Antifreeze proteins (AFPs) are a class of IBPs that have been documented in a number of cold-tolerant fish, insect, bacterial, fungal, and plant species, and this phenotype permits them to prevent and/or control ice crystal formation. Previously we examined the expression, ice binding affinity, and effect on cell viability during freeze-thaw cycling of a bacterial protein. This 54 kDa AFP (IBPv) was secreted by a bacterium within the family Flavobacteriaceae (strain 3519–10) that was isolated from a depth of ~3.5 km in the Vostok Ice Core. Based on the recombinant IBPv exhibiting TH of 2.2°C at a concentration of 53μM, it is categorized as a hyperactive AFP. According to primary sequence, IBPv was predicted to consist of two separate ice binding domains.

Each domain contains a six-loop right-handed β-helix (solenoid) with a triangular cross section, and an α-helix, which runs parallel on one side of the β-helix. However, no electron density was observed for the last 88 amino acids of the C-terminus. Each domain contains one intra-domain disulfide bond, namely C165-C226 in domain A and C244-C443 in domain B. Sometimes the ice binding regions also consist of well aligned side chains and even well aligned water molecules. In the IBPv structure, one flat plane was observed on the same surface for each domain as shown in Fig 1B and Fig 2, and they were not at the protein-protein contacts in the crystal. Site-directed mutagenesis confirmed that the proposed ice binding site for each domain is located at the same region on the β-helix for IBPv. Each domain of IBPv has two rows of water molecules on the IBS that form hydrogen bonds with the protein backbone, and more water molecules are found in the IBS of domain B compared to domain A. In the crystal structure of IBPv, a layer of ordered water molecules forms a water network that consists of several pentagonal and hexagonal ring on the IBS of domain B. However, no such water network is observed on the IBS of domain A, which is the weaker one in ice binding activity of the two domains, suggesting that the presence of water network is correlated with the ice binding activity and thus supporting the anchored clathrate water binding mechanism. Close molecular comparison of the two domains revealed that the bulky side chain of Leu 174 on the IBS of domain A may account for its inferior antifreeze activity.

>[2x]MQAPTLGAAANFALFTTAGAVTNTGLSHITGDVGTNNAASTNFGNVDGVMQDSNGATSAAAADLLIAYNLLNAAIPTATLAPLLGNGTTLTAGNYFIGQGASLSGTLTLDGGGNSNSVFIFKIQGALSSAANTQVLLTNGALACNVFWKVEGLVDLATNTVMKGNVVANNAAIVLQSGVSLEGRALSTTGAITVTGVTVRKPILCGSAVLTGPVAPNLGTVVCYTIFSGNGALTNAGITYVTGDVGTNVGLTTGFQADNVNGTIHSNPDTSTAQAALDLNNAYTYLNTLPTDIELLYPAAFGQNLVLTPHTYLLNAATVLNGKVTLDAQGNENAVFVIKINGALSTTVNASVELINGAIAKNVFWKVDGAVDLNDYTKFKGSVIGNNGAVIINTGVEIEGRVLSTSGGISTFGINAQMTPGCELLGTGSNTVAIQAAKFYPNPFSSVLNVTMEDLNGGSTLTIYNAAGSQVFSKVLSTKTTSLSMKLPAGVYFYQMIGKNGAKQAGKLIAKPHHHHHH>MQRARPGELVEVIMFRPTGKARVSNLDESMAMEFTDLRTRAMSSAAMIRQSVAAKTLLIENEDGKGSTRMEVQDFMKRFHMHASEDDKTGSPSTAWGTLRFPTKEATAPYLRLSVNDDPEDALLFVKAMLAQKYGETYDRPSLILSVTGGARNFTLPPRLETAIAKGLRLAAQRTNAWVVTGGTNTGVMKLTGQIMEALSKTQSHFIPPTIGIATYGVIIGGDDMTRGEPPKIGLEYEMHKKDPPKTTPLDDNHNLFLLVDDGSTNKFGKEIKFRAAFENAAGQAFAAPVVTIVVQGGPGTLGTALQAVRQGTPIVVVDGSGLAADVLAYAYNFMHNPLTRFKSYTIDDLRQKVAQTFNPKSSQQLTNLLDSALECVQDPNLVVVYSLQESGIDEFDDCILKAIFSSQGKLGNKLKQAMYFDQLDVAKRALSEASKNGQHNEIAACINDNLMAAMMHNKPHFVELYLGFDAKIYELKPSEEVAKTNITALDELPSFALAIEELYKREAKKPHSHVQRLVSLSNTDVLGRHYRVSTQRGDGTTRRIGRDLANTRAYNVLRMDQIFARLVSKDFSVNRDFTIYDSKYDKVPGIQFRRTAQASHMLFLWAICLDRFRMARHFWLIGDQSIINALVASRILERLSTHRALQGPHLAEERAKMQHNAKKFEELAVGVLGECHGSDSHMASEMLHSKNDMFNKKNAINIAYDAKSLAFLSHPATQSVINADWYGHLKSVTSFWAVLFAFFFPFFVLPFINFSEDHAEQQVEAPRDFFTDAPRSSHSANSTTSGAHRLRRKFAKFYSAPYTRFISDLLSHFVLCVVTSYFVLDKLEDTISAIEWILLVWFVALLLEELRQMIFCDGIAEYISDTWNRLDLIMITLFFVGFFTHASDPSNQDSKVVSKGIHAFLVVVLWLRFMRYYALSKNLGPKLIMMMEMMKDVSTFVFLLLIFLIGYGVAAQSLLSPDEDFSSRTFIGVLFRPYFQIYGELFLDDLNSEANCLGDTPFTECSRETVRMVPFFLAVYILGSNVLLVNLLIAMFNDTYMKVQEAAEDLWRKQNYELCAEYKDRPFLPAPFILLAHVHMLFMRLLRLCGVHTQEHEKIQDDETKRKITTFEELNTDKFLRRWERERQEMLEARVKMTNDNVVQAMGMMDQLLEHMISFRFSLDQQATKIKQEIRDDGLPSTEPTGLVSRTPSQPINRLNSAVAVHGHTAEAAEWYVPPEEYPKSGGVKRYLIDASMVPLSIMCPSYDPVEYTHPSVAAQPVWADPADPRKIKFNVKDEVNGKVVDRTSCHPSGISIDSNTGRPINPWGRTGMTGRGLLGKWGVNQAADTVVTRWKRSPDGSILERDGKKVLEFVAIQRQDNKMWAIPGGFVDNGEDVALTSGREFMEEALGMGTSADLMSAESKDSLAALFSSGTIVARIYCEDPRNTDNAWVETTCVNFHDESGRHAARLKLQGGDDAEHARWMMVHGGLNLFASHRTLLQHVTSALNAYF[4x]

We investigated a TRPM2 chanzyme from choanoflagellates that integrates two seemingly incompatible functions into a single peptide: a channel module activated by ADP-ribose with high open probability and an enzyme module (NUDT9-H domain) consuming ADP-ribose at a remarkably slow rate. Using time-resolved cryogenic-electron microscopy, we captured a complete series of structural snapshots of gating and catalytic cycles, revealing the coupling mechanism between channel gating and enzymatic activity. The slow kinetics of the NUDT9-H enzyme module confers a self-regulatory mechanism: ADPR binding triggers NUDT9-H tetramerization, promoting channel opening, while subsequent hydrolysis reduces local ADPR, inducing channel closure. The structures of srTRPM2 exhibit a characteristic TRPM architecture, from top to bottom, a transmembrane domain (TMD) layer containing the ion-conducting pore, a signal transduction layer consisting of MHR3/4 domain and the C-terminal rib helix, and an ADPR-sensing layer consisting of the N-terminal MHR1/2 domain and the C-terminal NUDT9-H domain.

The density of a representative bound cholesterol molecule is shown in the box. b, The ion-conducting pore in the apo (left) and Mg2+–ADPR-bound open (middle) states viewed parallel to the membrane, with plots of the pore radius along the pore axis (right). Before the onset of hydrolysis (substrate-bound state), both MHR1/2 and NUDT9-H domains are occupied by ADPR. Within NUDT9-H, the adenine group of ADPR is sandwiched by the indole group of W1264 and the phenyl group of F1372 via π–π stacking. Three Mg2+ cofactors (Mg1, Mg2 and Mg3) are bound between the two phosphate groups of ADPR and two acidic residues on the Nudix helix, E1386 and E1390. The extensive interactions between ADPR and the NUDT9-H domain strategically anchor both termini of the ADPR molecule, exposing only its α-phosphate (Pα) to solvent and making it readily accessible for nucleophilic attack. Indeed, we observed a putative water molecule bridging Mg2 and Mg3, as previously found in the crystal structure of NUDT5. On activation by Mg2+ ions, the water molecule is deprotonated by the catalytic base D1460 located in a loop close to the Nudix helix, and is poised for nucleophilic attack on the phosphorus atom of Pα.> HHHHHHATAVVRCRTRLARRVVAAVGPDGL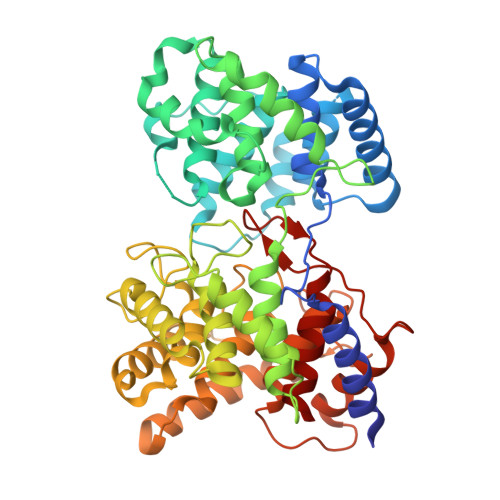LPAPCESRVLESALALALLTEERAEADATARLTAYLRTTLRTAPPDPFQCAVARAVLGGAGERGERVGDEGDMDAGTALDAGLDGFDHFTAGRKRLMFRTVLAALGATGFPAVPWEAYDTRPQQSWLHMEMKALKVLAAHGTGHPDVVRDEDWRALLPALEPGPAWECNNLAQLLALLALRHSPRHRPALGDVLKHVAGRLRPDGGMPFIDGMTVFTTAAAGLALSLLPAPPACVTPMADALALRRNPDGGYGFHSGVAQSDVDDTCYVLEFLRRAAPDRHRTAVAEAEGYLLALRNPDGGFPTFARGTSSEIAMTAAAASALAHDPDRREEVDEAVRYVVRHQRPDGTFERSWSRNATNAVFRAVLALTGVAAHGEERRSRARAAERALAHLAATQNGDGGWGHAEAEPSDPISTAYAVIALARGPRARPGGPLDRALAYLVERQHPDGGYRSRPDQAGPRPLLYDVPALADVFVLLALAHAT> MDGPYLQILEQPKQRGFRFRYVCEGPSHGGLPGASSEKNKKSYPQVKICNYVGPAKVIVQLVTNGKNIHLHAHS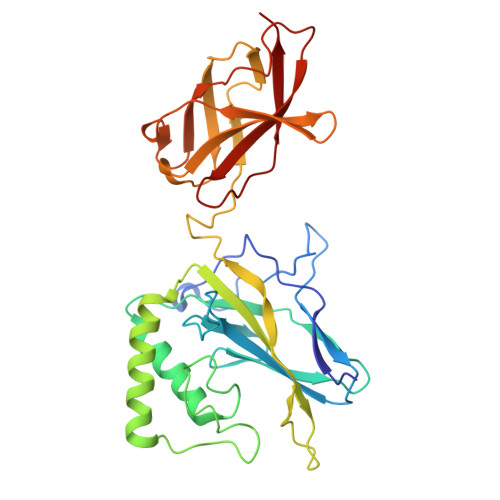LVGKHCEDGICTVTAGPKDMVVGFANLGILHVTKKKVFETLEARMTEACIRGYNPGLLVHPDLAYLQAEGGGDRQLGDREKELIRQAALQQTKEMDLSVVRLMFTAFLPDSTGSFTRRLEPVVSDAIYDSKAPNASNLKIVRMDRTAGCVTGGEEIYLLCDKVQKDDIQIRFYEEEENGGVWEGFGDFSPTDVHRQFAIVFKTPKYKDINITKPASVFVQLRRKSDLETSEPKPFLYYPE>MTSMTQSLREVIKAMTKARNFERVLGKITLVSAAPGKVICEMKVEEEHTNAIGTLHGGLTATLVDNISTMALLC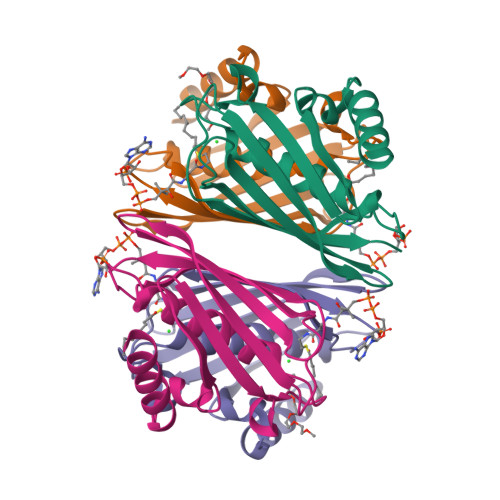TERGAPGVSVDMNITYMSPAKLGEDIVITAHVLKQGKTLAFTSVDLTNKATGKLIAQGRHTKHLGNLEHHHHHH[8x]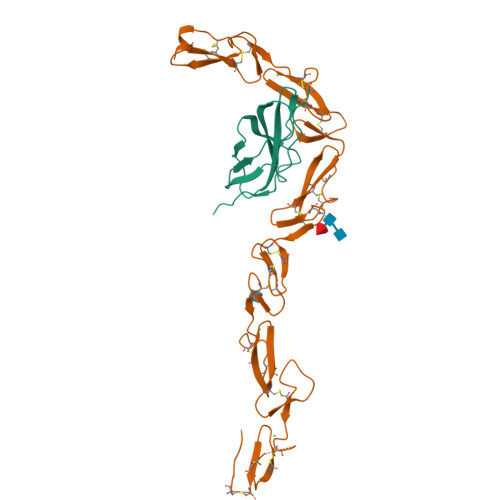> AEPSSPPGAPSQPVVTEITKNSITLTWKPNPQTGAAVTSYVIEAFSPAAGNTWRTVADGVQLETHTVSGLQPNTIYLFLVRAVGAWGLSEPSPVSEPVRTQDSSPSRPVEDPWR;> AGYDFCSERHNCMENSICRNLNDRAVCSCRDGFRALREDNAYCEDIDECAEGRHYCRENTMCVNTPGSFMCICKTGYIRIDDYSCTEHDECITNQHNCDENALCFNTVGGHNCVCKPGYTGNGTTCKAFCKDGCRNGGACIAANVCACPQGFTGPSCETDIDECSDGFVQCDSRANCINLPGWYHCECRDGYHDNGMFSPSGESCEDIDECGTGRHSCANDTICFNLDGGYDCRCPHGKNCTGHHHHHH> MAHHHHHHMDAATTRAGLTDLKFRLVRESFADAVSWVAKNLPTRPAVPVLSGVLLTGSDEGLTISGFDYEVSAEVRVPAEIASPGTVLVSGRLLS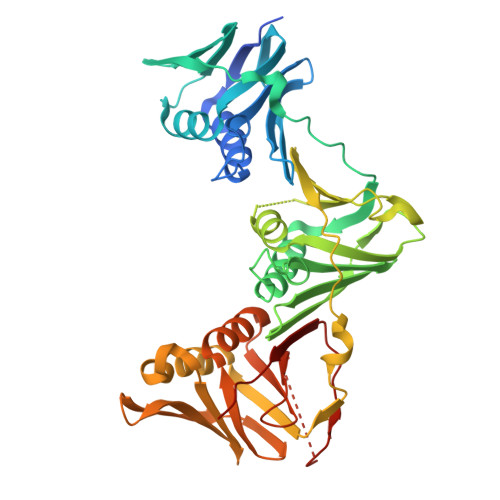DITRALPNKPVDFYVDGNRVALTCGNARFSLPTMAVEDYPTLPTLPEDTGTLPAELFSEAIGQVAIAAGRDDTLPMLTGIRVEISGEKVVLAATDRFRLAVRELTWNALSPDIEAAVLVPAKTLGEAAKANTDGSEVRLSLGAGMGVGKDGLLGISGDGKRSTTRLLDAEFPKFRQLLPAEHTAVASADVAELTEAIKLVALVADRGAQVRMEFADGMLRLSAGADDVGRAEEDIAVEFAGQPLTIAFNPTYLIDGLASLHSERVSFGFTTPGKPALLRPASAEDRIVSGPGDQGPFAAVPTDYVYLLMPVRLPG> 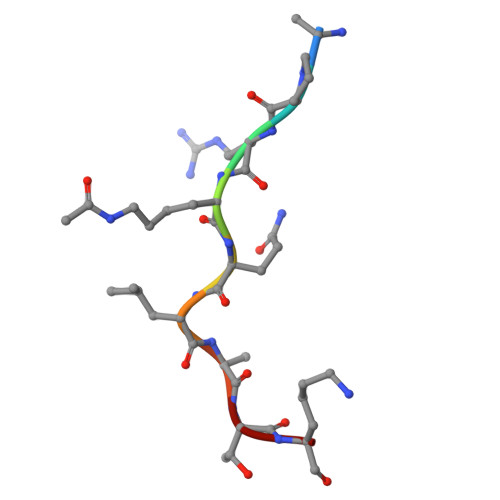APRKQLATK2-ethyl-N-(2-hydroxyphenyl)butanamide 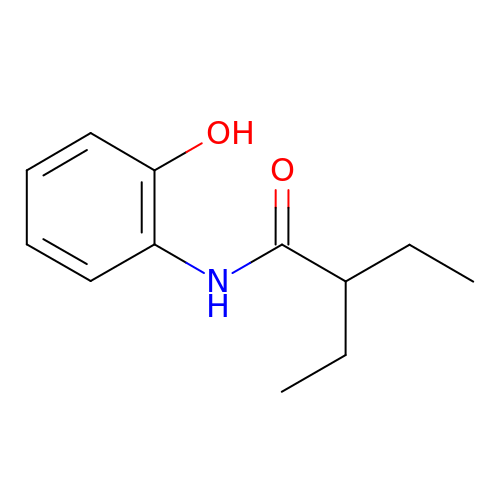| C12 H17 N O2 | ZHIXKMXOQAKAKN-UHFFFAOYSA-N>MADKIKDAKIIFVVGGPGSGKGTQCEKIVAKYGYTHLSSGDLLRAEVSSGSERGKQLQAIMQKGELVPLDTVLDMIKDAMIAKADVSKGYLIDGYPREVKQGEEFEKKIGKPCLLLYIDAKGETMVKRLMKRGETSGRADDNEETIKKRLDLYYKATEPVIAFYEGRGIVRKIDSELPVDEVFKQVSTAIDAL[2x]

AK is a small enzyme that catalyzes a reversible phosphoryl transfer reaction between ATP/AMP and two ADPs. The structures comprised the characteristic three-domain arrangement: the CORE (residues 1–38, 69–136, and 143–193), AMPbind (residues 39–68), and LID (residues 137–142) domains. The static CORE domain provides substrate-binding sites, and the dynamic AMPbind and LID domains close over the AMP and ATP sites, respectively, upon substrate binding. AK is a small protein that undergoes relatively large conformational changes upon substrate binding and product release, and has long been used as a model system for studying connections between structure, function, and dynamics.

To confirm that thermal stabilization caused by the Val-to-Ile mutations resulted from the optimized hydrophobic CORE packing, we determined the crystal structure of a V28I/V118I/V173I mutant of AKNc. The Tm value of the V28I/V118I/V173I mutant was 11.3 °C higher than that of the WT AKNc, and was identical to that of AKDr, the most thermally stable homologue of the three tropical AKs. The overall tertiary structure of the mutant was essentially identical to that of the WT. In the mutant structure, the conformations of the residues neighboring the mutated Ile28 residue were almost indistinguishable from those around Val28 in the WT AKNc structure. This allows the added terminal methyl group (Cδ1) of the Ile28 side chain to interact hydrophobically with other residues in the CORE domain—such as Val13, Cys25, Leu91, Leu116, Val186, and Ile190—indicating the enhancement of the hydrophobic packing by the V28I mutation. The conformation of Ile118 was essentially identical to that of Val118 in the WT structure, with the exception of the extra methyl group (Cδ1) in its side chain, which makes additional hydrophobic contacts with Val13, Gln24, Leu116, and Val186 in β1, α1, β4, and α9, respectively, in the mutant structure. In contrast, the side chain conformation of the mutated Ile173 residue was distinct from that of Val173 in WT AKNc. The χ1 dihedral angle along the bond between the Cα and Cβ atoms of Ile173 was rotated ~120° relative to that of Val173 in the WT AKNc structure. The flipped side chain of Ile173 interacts hydrophobically with residues in β4, β5, and α9, including Leu116, Arg171, Val182, Val186, and Ala189. It seems that the improvement in hydrophobic CORE packing by the Val-to-Ile mutations increased the structural stability at high temperatures and decreased the catalytic activity at low temperatures.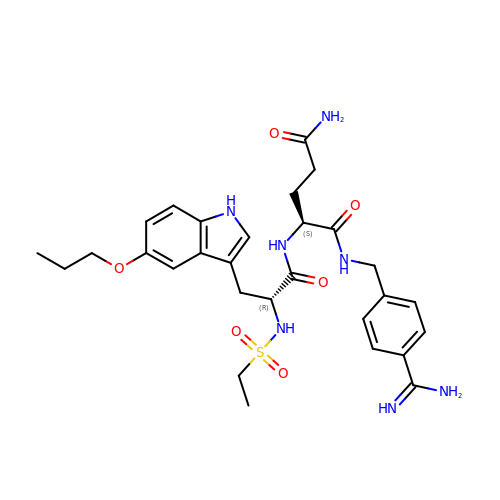N-(ETHYLSULFONYL)-5-PROPOXY-L-TRYPTOPHYL-N~1~-{4-[AMINO(IMINO)METHYL]BENZYL}-L-GLUTAMAMIDE | C29 H39 N7 O6 S | UHMORXPPNXDKHY-LOSJGSFVSA-N> MGHHHHHHHHHHSSGHENLYFQGHMANRNVEKLASIDAQLRLLVPGKVSEDDKLVEYDALLLDKFLDILQDLHGEDLKEAVQQCYELSAEYEGKHDPKKLEELGSLLTSLDTGDSIVIAKAFSHMLNLANLAEELQIAYRRRIKLKSGDFADEANATTESDIEETFKRLVHKLNKSPEEVFDALKNQTVELVLTAHPTQSVRRSLLQKHGRIRNCLAQLYAKDITPDDKQELDEALHREIQAAFRTDEIRRTPPTPQDEMRAGMSYFHETIWKGVPKFLRRVDTALKNIGINERFPYNAPLIQFSSWMGGDRDGNPRVTPEVTRDVCLLARMMTSNMYFSQIEDLMIEMSMWRCNSELRVRAEELYRTARKDVKHYIEFWKRIPPNQPYRVILGDVRDKLYNTRERSRHLLVDGKSDIPDEAVYTNVEQLLEPLELCYRSLCDCGDHVIADGSLLDFLRQVSTFGLSLVKLDIRQESDRHTEVLDAITQHLGIGSYREWSEEKRQEWLLAELSGKRPLIGPDLPKTEEVKDCLDTFKVLAELPSDCFGAYIISMATSTSDVLAVELLQREYHIKHPLRVVPLFEKLADLEAAPAAMTRLFSMDWYRNRIDGKQEVMIGYSDSGKDAGRFSAAWQLYKTQEQIVKIAKEFGVKLVIFHGRGGTVGRGGGPTHLALLSQPPDTINGSLRVTVQGEVIEQSFGEEHLCFRTLQRFCAATLEHGMNPPISPRPEWRELMDQMAVVATEEYRSVVFKEPRFVEYFRLATPELEFGRKNIGSRPSKRKPSGGI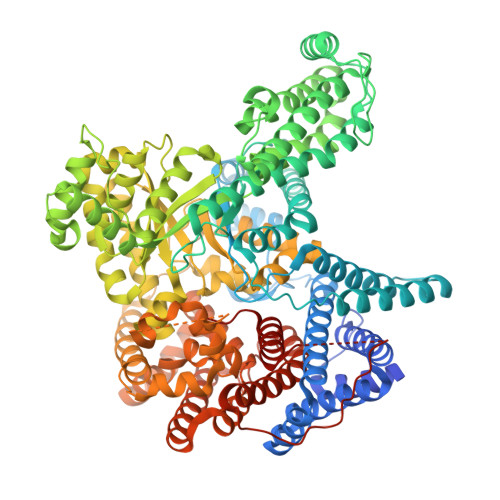ESLRAIPWIFSWTQTRFHLPVWLGFGAAFKHAIQKDSKNLQMLQEMYKTWPFFRVTIDLVEMVFAKGNPGIAALNDKLLVSEDLRPFGESLRANYEETKNYLLKIAGHKDLLEGDPYLKQGIRLRDPYITTLNVCQAYTLKRIRDPNYHVTLRPHISKEYAAEPSKPADELIHLNPTSEYAPGLEDTLILTMKGIAAGMQNTG>[4x]HHASAKTYTLTDYLKNTYRLKLYSLRWISDHEYLYKQENNILVFNAEYGNSSVFLENSTFDEFGHSINDYSISPDGQFILLEYNYVKQWRHSYTASYDIYDLNKRQLITEERIPNNTQWVTWSPVGHKLAYVWNNDIYVKIEPNLPSYRITWTGKEDIIYNGITDWVYEEEVFSAYSALWWSPNGTF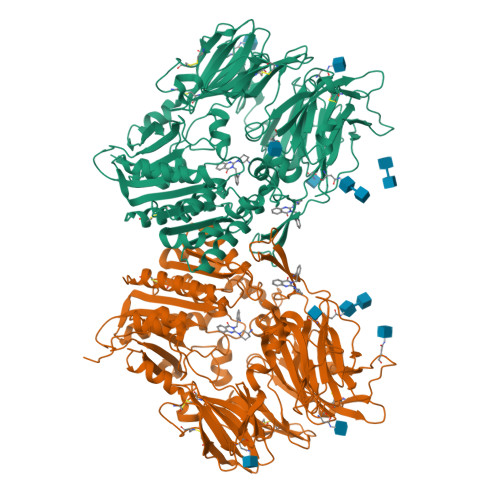LAYAQFNDTEVPLIEYSFYSDESLQYPKTVRVPYPKAGAVNPTVKFFVVNTDSLSSVTNATSIQITAPASMLIGDHYLCDVTWATQERISLQWLRRIQNYSVMDICDYDESSGRWNCLVARQHIEMSTTGWVGRFRPSEPHFTLDGNSFYKIISNEEGYRHICYFQIDKKDCTFITKGTWEVIGIEALTSDYLYYISNEYKGMPGGRNLYKIQLSDYTKVTCLSCELNPERCQYYSVSFSKEAKYYQLRCSGPGLPLYTLHSSVNDKGLRVLEDNSALDKMLQNVQMPSKKLDFIILNETKFWYQMILPPHFDKSKKYPLLLDVYAGPCSQKADTVFRLNWATYLASTENIIVASFDGRGSGYQGDKIMHAINRRLGTFEVEDQIEAARQFSKMGFVDNKRIAIWGWSYGGYVTSMVLGSGSGVFKCGIAVAPVSRWEYYDSVYTERYMGLPTPEDNLDHYRNSTVMSRAENFKQVEYLLIHGTADDNVHFQQSAQISKALVDVGVDFQAMWYTDEDHGIASSTAHQHIYTHMSHFIKQCFSLP> SHMNSEILNNIILNLRYRDNNLIDLSGYGANVEVYDGVELNDKNQFKLTSSTNSEIRVTQNQNIIFNSMFLDFSVSFWIRIPKYKNDGIQNYIHNEYTIINCIKNNSGWKISIRGNRIIWTLTDINGKTKSVFFEYSIREDISDYINRWFFVTITNNSDNAKIYINGKLESN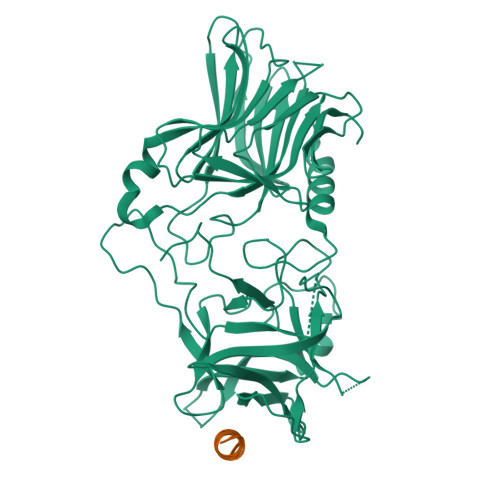IDIKDIGEVIANGEIIFKLDGDIDRTQFIWMKYFSIFNTELSQSNIKEIYKIQSYSEYLKDFWGNPLMYNKEYYMFNAGNKNSYIKLKKDSSVGEILTRSKYNQNSNYINYRNLYIGEKFIIRRKSNSQSINDDIVRKEDYIYLDFFNSNREWRVYAYKDFKEEEKKLFLANIYDSNEFYKTIQIKEYDEQPTYSCQLLFKKDEESTDEIGLIGIHRFYESGIVLKDYKNYFCISKWYLKEVKRKPYNPNLGCNWQFIPKDEGWIE;> GEGKEDAFSKLKEKFMNELHK> MELKHSI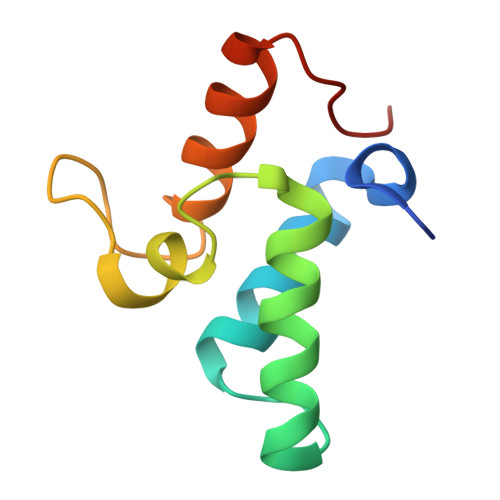SDYTEAEFLEFVKKIARAEGATECDDNKLVREFERLTEHPDGSDLIYYPRDDREDSPEGIVKEIKEWRAANGKSGFKQG> MLRNTFTRAGGLSRITSVRFAQTHALSNAAVMDLQSRWENMPSTEQQDIVSKLSERQKLPWAQLTEPEKQAVWYISYGEWGPRRPVLNKGDSSFIA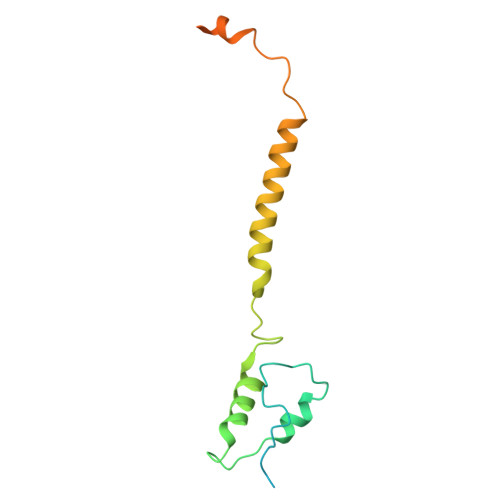KGVAAGLLFSVGLFAVVRMAGGQDAKTMNKEWQLKSDEYLKSKNANPWGGYSQVQSK> LPICPGGAARCQVTLRDLFDRAVVLSHYIHNLSSEMFSEFDKRYTHGRGFITKAINSCHTSSLATPEDKEQAQQMNQKDFLSLIVSILRSWNEPLYHLVTEVRGMQEAPEAILSKAVEIEEQTKRLLEGMELIVSQVHPETKENEIYPVWSGLPSLQMADEESRLSAYYNLLHCLRRDSHKIDNYLKLLKCRIIHNNNC;>[2x]QSPPG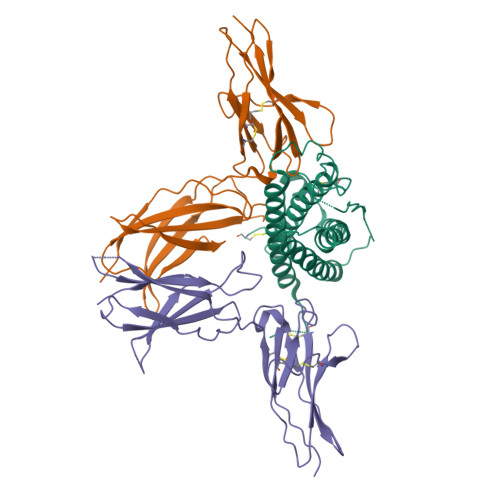KPEIHKCRSPDKETFTCWWNPGTDGGLPTNYSLTYSKEGEKTTYECPDYKTSGPNSCFFSKQYTSIWKIYIITVNATNQMGSSSSDPLYVDVTYIVEPEPPRNLTLEVKQLKDKKTYLWVKWSPPTITDVKTGWFTMEYEIRLKPEEAEEWEIHFTGHQTQFKVFDLYPGQKYLVQTRCKPDHGYWSRWSQESSVEMPNDFTLKDRSRSHHHHHH> GPGGSGEEDRSCTLANNFA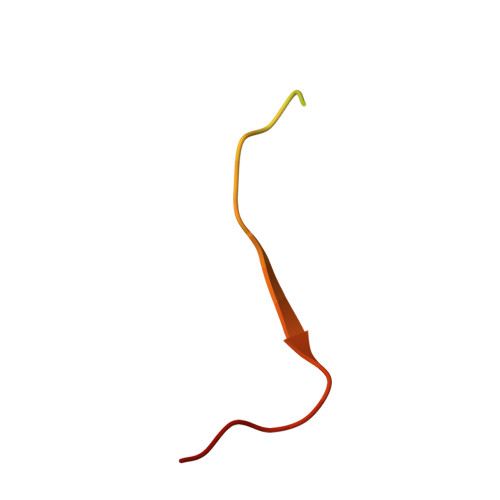RSFTLMLRYNGPPPT(2-nitro-4-{[(3S)-1-{[4-(trifluoromethoxy)phenyl]methyl}pyrrolidin-3-yl]amino}phenyl)methanol | 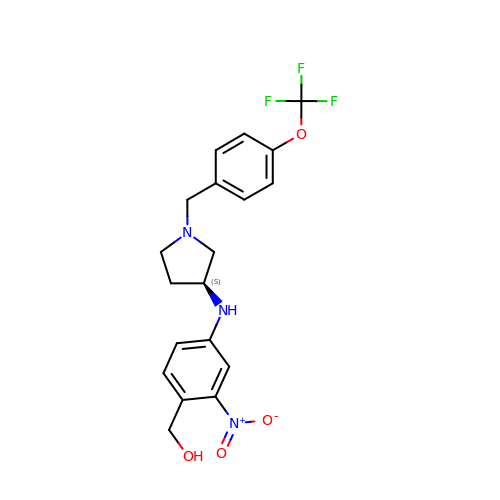C19 H20 F3 N3 O4 | BFPNKWNLPSACDB-INIZCTEOSA-N(3-chlorophenyl) 6-methyl-2-oxidanylidene-chromene-3-carboxylate 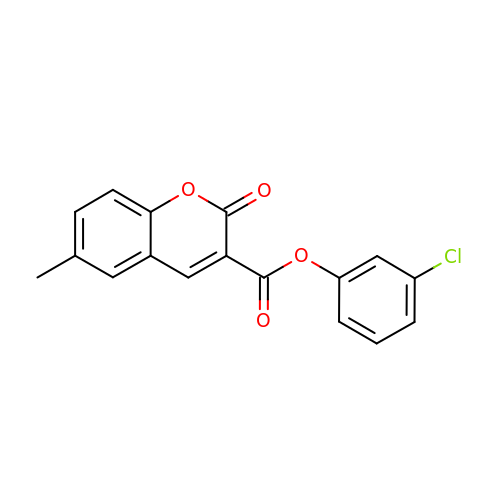| C17 H11 Cl O4 | BZDNWZYKPRTPIF-UHFFFAOYSA-N> MEPVGCCGECRGSSVDPRSTFVLSNLAEVVERVLTFLPAKALLRVACVCRLWRECVRRVLRTHRSVTWISAGLAEAGHLEGHCLVRVVAEELENVRILPHTVLYMADSETFISLEECRGHKRARKRTSMETALALEKLFPKQCQVLGIVTPGIVVTPMGSGSNRPQEIEIGESGFALLFPQIEGIKIQPFHFIKDPKNLTLERHQLTEVGLLDNPELRVVLVFGYNCCKVGASNYLQQVVSTFSDMNIILAGGQVDNLSSLTSEKNPLDIDASGVVGLSFSGHRIQSATVLLNEDVSDEKTAEAAMQRLKAANIPEHNTIGFMFACVGRGFQYYRAKGNVEADAFRKFFPSVPLFGFF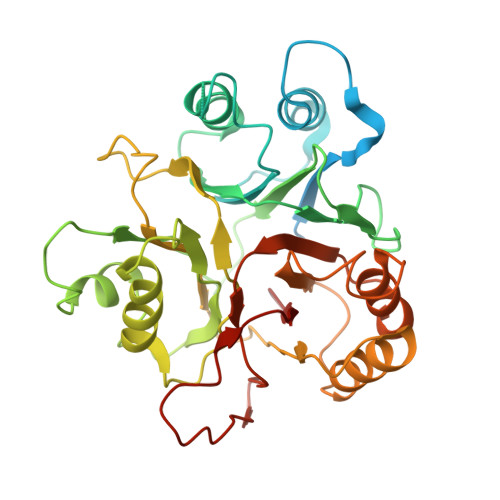GNGEIGCDRIVTGNFILRKCNEVKDDDLFHSYTTIMALIHLGSSK> MTDTPFIRPDMKAFLEAIAAMAGPTLAEMTLEEARASYVALHGMADRPARELAVIRNLSCPGPAGDIPLRLYDARESREAGPVITFYHGGGFVIGDLDTHHNLCTEIAALMDLPVVAVDYRLAPEHPFPAAIEDCEAATRWVASSPSELGRTASGVIPIGDSAGGNATIVVSQLLGAKPADVPVVLQVPIFPLASDAVGSASLAAFAEGFVLTKASIEFFDTAYKADRADPRGFPILGDHTAAPPTIVATASLDPIR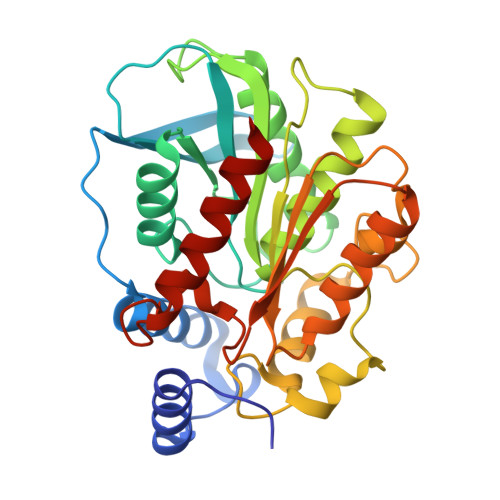DSGRDYAKALVEAGRDVVYLEMEGVTHSFTNIRAAVPSTQGDLERIIAAMKMMLGTA> MTALTESSTSKFVKINEKGFSDFNIHYNEAGNGETVIMLHGGGPGAGGWSNYYRNVGPFVDAGYRVILKDSPGFNKSDAVVMDEQRGLVNARAVKGLMDALDIDRAHLVGNAMGGATALNFALEYPDRIGKLILMGPGGLGPSMFAPMPMEGIKLLFKLYAEPSYETLKQMLQVFLYDQSLITEELLQGRWEAIQRQPEHLKNFLISAQKAPLSTWDVTARLGEIKAKTFITWGRDDRFVP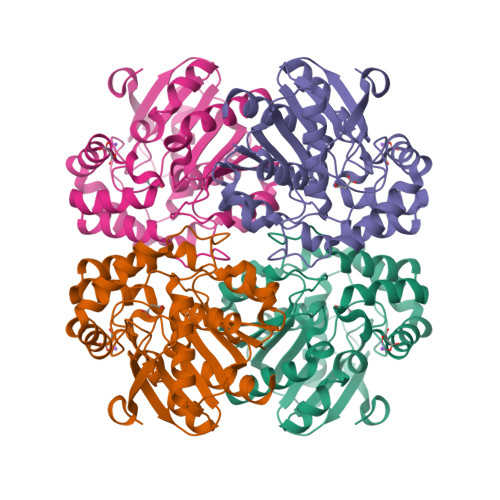LDHGLKLLWNIDDARLHVFSKCGAWAQWEHADEFNRLVIDFLRHA>[2x]GHMFSIQQPLLVFS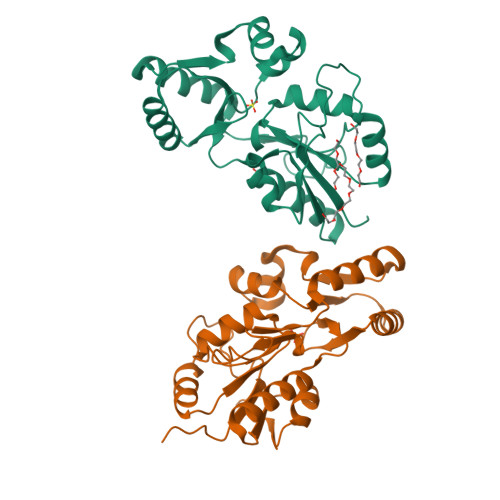DLDGTLLDSHSYDWQPAAPWLTRLREANVPVILCSSKTSAEMLYLQKTLGLQGLPLIAENGAVIQLAEQWQEIDGFPRIISGISHGEISLVLNTLREKEHFKFTTFDDVDDATIAEWTGLSRSQAALTQLHEASVTLIWRDSDERMAQFTARLNELGLQFMQGARFWHVLDASAGKDQAANWIIATYQQLSGKRPTTLGLGDGPNDAPLLEVMDYAVIVKGLNREGVHLHDEDPARVWRTQREGPEGWREGLDHFFSARGS> MIEPIKRTQVVTQTIHYRYEDGAVAHDDHVVSLIFTQSGKRDLTNGKEIWDSKWSLTQTFEALPSPVIIGYTADKPMVG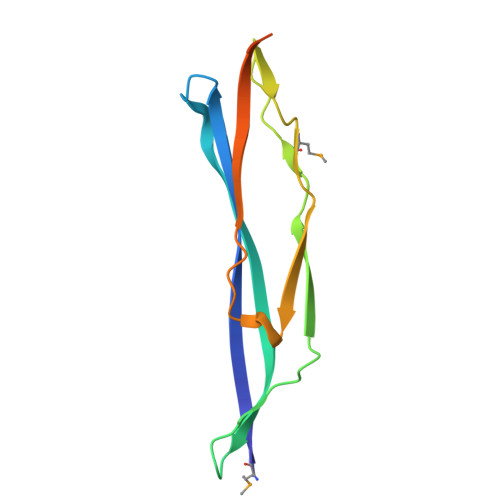PDEVTVDSKNFLDKQNREETVIYSANTITQNKKDGLEHHHHHH> MKELIYIEEPSILFAHGQKCTDPRDGLALFGPLNQIYGIKSGVVGTQKGLQIFKSYLDKIQKPIYNHNNITRPMFPGFEAVFGCKWESQNIVFKEITDEEIRRYLFNASTHKRTYDLVTLFNDKIITANKNDEERVDVWFVIVPEEIYKYCRPNSVLPNELVQTKSLISKSKAKSFRYTPTLFEEFNKKLKEVEKEAKTYNYDAQFHDQLKARLLEHTIPTQILRESTLAWRDFKNTFGAPIRDFSKIEGHLAWTISTAAYYKAGGKPWKLGDIRPGVCYLGLVYKKIEKSKNPQNACCAAQMFLDNGDGTVFKGEVGPWYNPEKGEYHLKPKEAKALLTQALESYKEQNKSYPKEVFIHARTRFNDEEWNAFNEVTPKNTNLVGVTITKSKPLKLYKTEGAFPIMRGNAYIVDEKKAFLWTLGFVPKLQSTLSMEVPNPIFIEINKGEAEIQQVLKDIL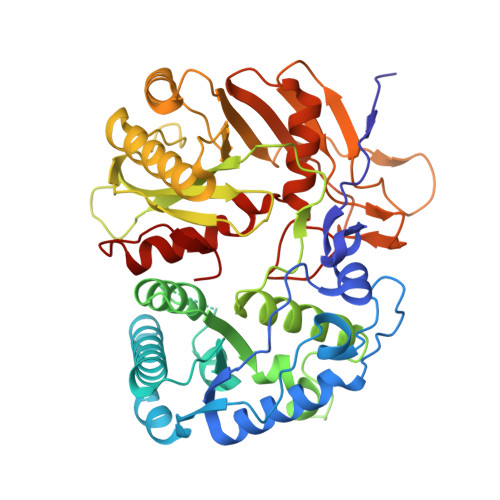ALTKLNYNACIYADGEPVTLRFANKIGEILTASTEIKTPPLAFKYYI> QVTPRPEAAPGARPGFRAPARIISPEIMPDNKVTFRVYSKDASKVTITGEWQTGPGGVEELVKNDTGMFSITVGPLKPELYAYNFTVDGVKALDANNVQVRRDGTNYQNFFIIPGPESDLYFHKNNVPHGTVTKVWYKSSVIGFDRRMYVYTPAGYEGDTQRYPVFYLLHGAGGDEDAWTNMGRTAQIMDNLIAQGKAK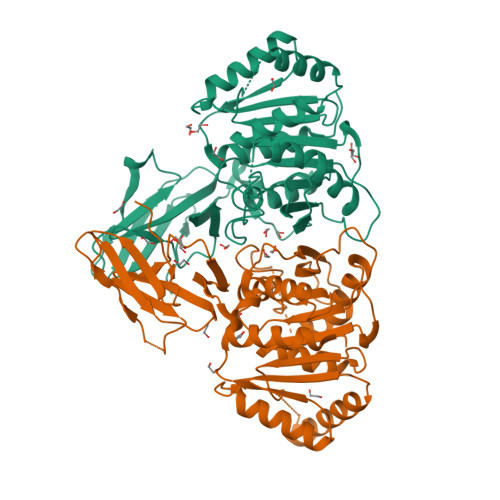PMIVVMTNGNANQAGAQNEVPPVPVTQGQQGIPSGSGMTGKFEEHLVKDVVPFIEKNFRALTGKDNRAIAGLSMGGGHTQTITNDNPGMFSYIGVFSMGIMAGRQQGADAEKIEKERDAKIEALKKSGYKLYWIACGKDDFVYQSALTLRNTLDKHNFKYVYRESTGGHTWANWRIYLSEFAPMLFKLL;> QVTPRPEAAPGARPGFRAPARIISPEIMPDNKVTFRVYSKDASKVTITGEWQTGPGGVEELVKNDTGMFSITVGPLKPELYAYNFTVDGVKALDANNVQVRRDGTNYQNFFIIPGPESDLYFHKNNVPHGTVTKVWYKSSVIGFDRRMYVYTPAGYEGDTQRYPVFYLLHGAGGDEDAWTNMGRTAQIMDNLIAQGKAKPMIVVMTNGNANQAGAQNEVPPVPVTQGQQGIPSGSGMTGKFEEHLVKDVVPFIEKNFRALTGKDNRAIAGLSMGGGHTQTITNDNPGMFSYIGVFSMGIMAGRQQGGDAEKIEKERDAKIEALKKSGYKLYWIACGKDDFVYQSALTLRNTLDKHNFKYVYRESTGGHTWANWRIYLSEFAPMLFKLL1-(adamantan-1-yl)-2-(1H-imidazol-1-yl)ethanone | 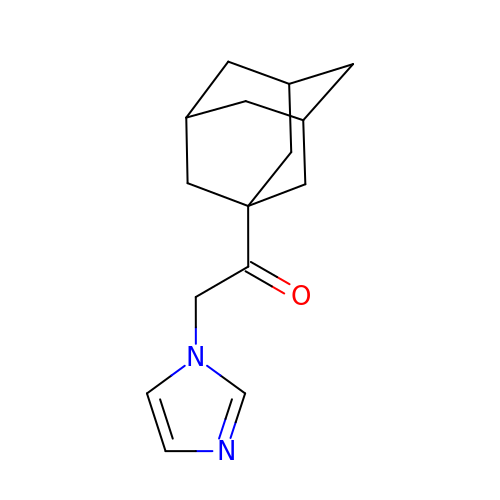C15 H20 N2 O | BBCQJSMDKDHVKG-BVMXXOESSA-N The main components of the system are transmembrane chemotaxis receptors called methyl-accepting chemotaxis proteins (MCPs), the histidine kinase CheA, and the adapter protein CheW. CheA functions as a dimer and possesses five domains (P1-P5) with distinct roles in autophosphorylation and array integration. The P1 domain is the phosphate substrate domain, P2 interacts with response regulators, P3 is the dimerization domain, P4 binds ATP, and P5 interacts with CheW. Here, we used cryo-ET to examine the in vivo array structure of the pathogenic spirochete Treponema denticola (Td), which possesses the highest native membrane curvature of any bacterial species examined for its chemotaxis system so far4,7.

Sequence alignments of Td CheA with CheA homologs from a variety of model bacteria with previously characterized chemotaxis systems indicate that, in Td CheA, an additional ~50 residues join the canonical dimerization domain (P3) helices. Analysis of non-redundant P3 domains from all CheA classes reveal general sequence conservation in the canonical helices but highly divergent sequences at these additional residues. Furthermore, CheA-F2 proteins contain the most residues in this non-conserved region. Interestingly, aromatic residues (Phe, Tyr) cluster near the helix breakages, and unusual core packing of these residues allows for maintenance of a coiled-coil register despite a disruption of helical heptad repetition in the C-terminal helix. The net result is a distortion in the alignment of the hairpin tip, the consequence of which is currently unknown. Different orientations of Tyr83 in the two subunits produce asymmetry in the added tip region. However, a linear arrangement of CheA is present that generates “strands” of rings interlinked by the CheA dimerization domain (P3). Furthermore, the Td CheA P3 domain is clearly discernible in the sub-tomogram averages, which has not been previously observed in vivo. As the CheA:CheW rings have to undergo substantial bending to accommodate the baseplate curvature, the elongated P3 domain may have evolved to stabilize CheA dimerization by increasing the interface area. Because of the high membrane curvature, the receptor trimer-of-dimer modules are expected to be further splayed, and the elongated P3 may compensate for the increased distance between receptors and P3.

>[2x]SILRVDANRIDYLLNLVSETVITKASLNQSTIEFAELYDKFQNSSTIYKDKTRRLLDKMPEYLEKIQQGYDINSIKQDVLNEYSSLLEVFGDFDSLMKAAVTKFKSSSQNLGRISGELQEGVMKIRMVP>[8x]EACKFLHQERMDVCETHLHWHTVAKETCSEKSTNLHDYGML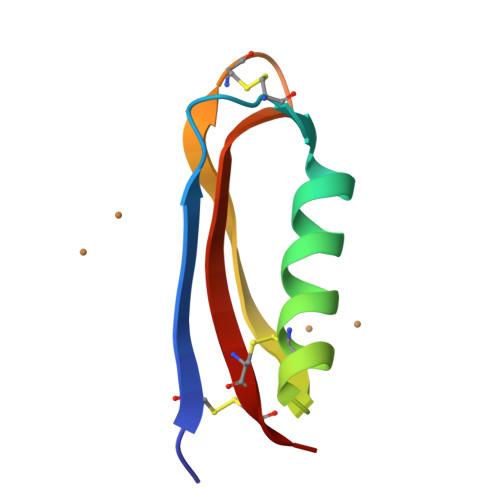LPCGIDKFRGVEFVCCPL> MASPDEDNPGILYNGRFDFSDPNGPKCAWSGSNVELNFYGTEASVTIKSGGENWFQAIVDGNPLPPFSVNATTSTVKLVSGLAEGAHHLVLWKRTEASLGEVQFLGFDFGSGKLLAAPKPLERKIEFIGDSITCAYGNEGTSKEQSFTPKNENSYMSYAAITARNLNASANMIAWSGIGLTMNYGGAPGPLIMDRYPYTLPYSGVRWDFSKYVPQVVVINLGTNDFSTSFADKTKFVTAYKNLISEVRRNYPDAHIFCCVGPMLWGTGLDLCRSYVTEVVNDCNRSGDL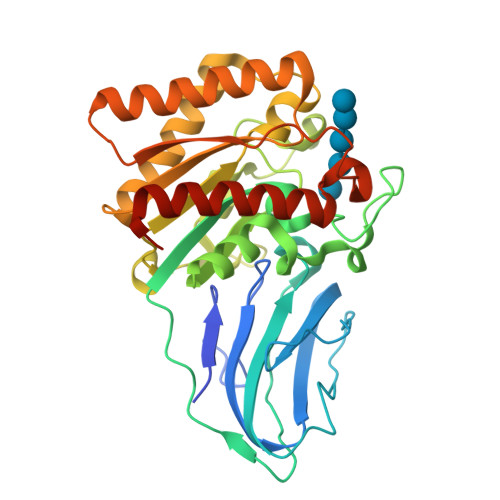KVYFVEFPQQDGSTGYGEDWHPSIATHQLMAERLTAEIKNKLGWLEHHHHHH(2S)-2-{[(AMINOMETHYL)(DIHYDROXY)SILYL]METHYL}-4-METHYLPENTANAL 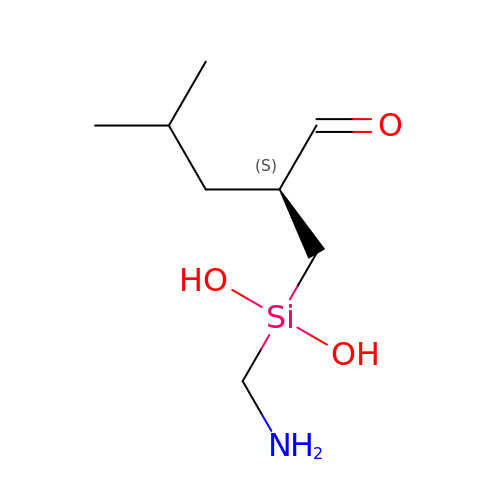| C8 H19 N O3 Si | ZZKRIEGAOOCWBS-QMMMGPOBSA-N> RAKKPRKART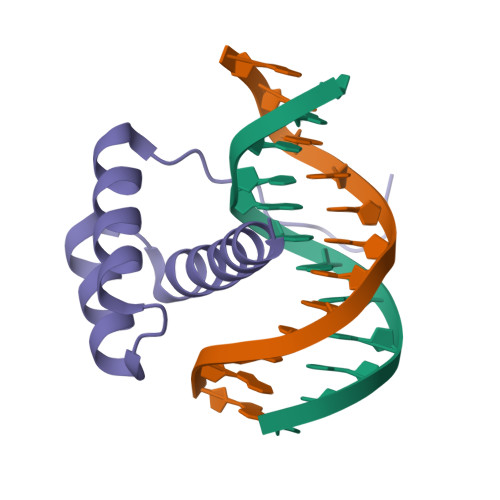AFSDHQLNQLERSFERQKYLSVQDRMDLAAALNLTDTQVKTWYQNRRTKWKRQTAV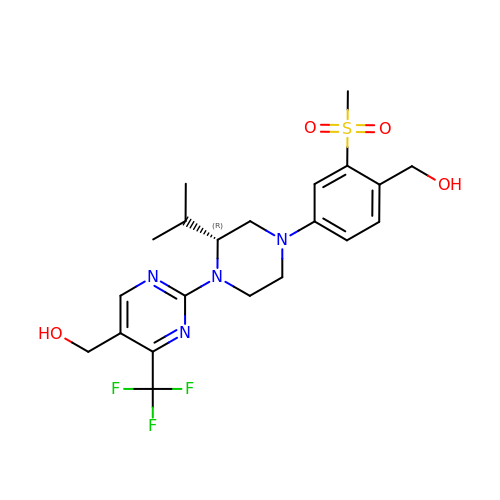{2-[(2R)-4-[4-(hydroxymethyl)-3-(methylsulfonyl)phenyl]-2-(propan-2-yl)piperazin-1-yl]-4-(trifluoromethyl)pyrimidin-5-yl}methanol | C21 H27 F3 N4 O4 S | FPVIRRAMNBCEDK-KRWDZBQOSA-N>[2x]MTDLKASSLRALKLMDLTTLNDDDTDEKVIALCHQAKTPVGNTAAICIYPRFIPIARKTLKEQGTPEIRIATVTNFPHGNDDIDIALAETRAAIAYGADEVDVVFPYRALMAGNEQVGFDLV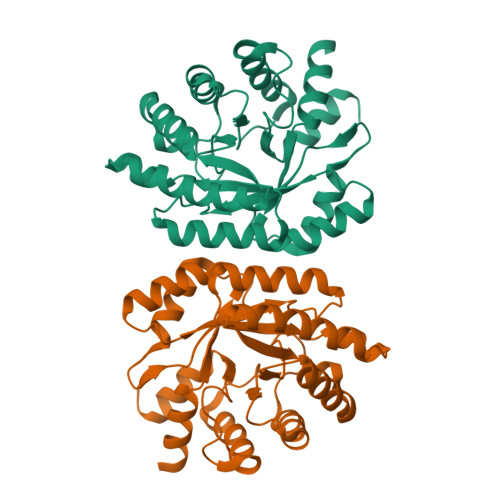KACKEACAAANVLLKVIIETGELKDEALIRKASEISIKAGADFIKTSTGKVAVNATPESARIMMEVIRDMGVEKTVGFKPAGGVRTAEDAQKYLAIADELFGADWADARHYRFGASSLLASLLKALGH> KETAAAKFERQHMDSX;>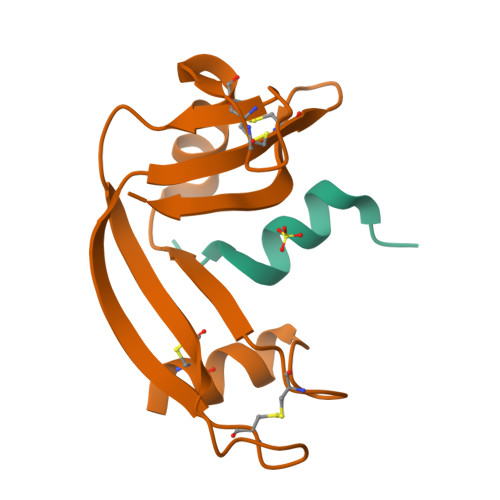 SSSNYCNQMMKSRNLTKDRCKPVNTFVHESLADVQAVCSQKNVACKNGQTNCYQSYSTMSITDCRETGSSKYPNCAYKTTQANKHIIVACEGNPYVPVHFDASV2-phenoxy-1-phenyl-3-(piperazin-1-ylcarbonyl)-1H-indole | C25 H23 N3 O2 | 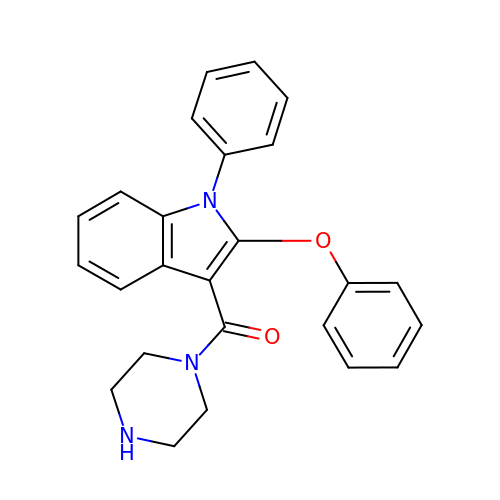PAQQZWUEZAUGRI-UHFFFAOYSA-N> ASPSSELRRALEANEFIPYYQPLSPGQGGRWIGVEVLMRWRHPREGLIRPDLFIPFAERSGLIVPMTRALMRQVAEDLGGHAGKLEPGFHIGFNISATHCHELALVDDCRELLAAFPPGHITLVLELTERELIESSEVTDRLFDELHALGVKIAIDDFGTGHSSLAYLRKFQVDCLKIDQSFVARIGIDTLSGHILDSIVELSAKLDLDIVAEGVETPEQRDYLAARGVDYLQGYLIGRPMPLESLLSSLTVQEGQ;> SPSSELRRALEANEFIPYYQPLSPGQGGRWIGVEVLMRWRHPREGLIRPDLFIPFAERSGLIVPMTRALMRQVAEDLGGHAGKLEPGFHIGF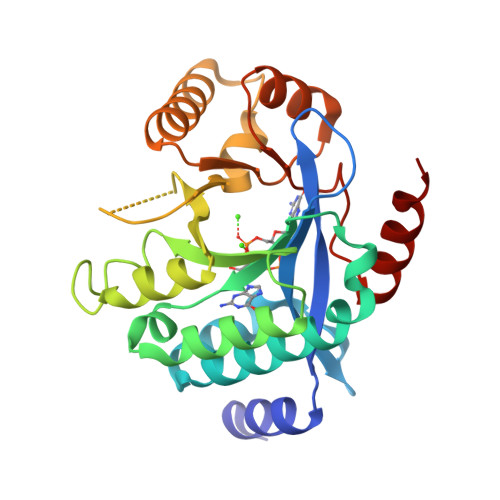NISATHCHELALVDDCRELLAAFPPGHITLVLELTERELIESSEVTDRLFDELHALGVKIAIDDFGTGHSSLAYLRKFQVDCLKIDQSFVARIGIDTLSGHILDSIVELSAKLDLDIVAEGVETPEQRDYLAARGVDYLQGYLIGRPMPLESLLSSLTVQEG>SNAMKKFSVVIAGGGSTFTPGIVLMLLANQDRFPLRSLKFYDNDGARQETIAEACKVILKEQAPEIEFSYTTDPQAAFTDVDFVMAHIRVGKYPMREQDEKIPLRHGVLGQETCGPGGIAYGMRSIGGVLELVDYMEKYSPNAWMLNYSNPAAIVAEATRRLRPNAKILNICDMPIGIEGRMAQIVGLKDRKQMRVRYYGLNHFGWWTSIEDLDGNDLMPKLREYVAKYGYVPPSNDPHTEASWNDTFAKAKDVQALDPQTMPNTYLKYYLFPDYVVAHSNPERTRANEVMDHREKNVFSACRAIIAAGKSTAGDLEIDEHASYIVDLATAIAFNTQERMLLIVPNNGAIHNFDADAMVEIPCLVGHNGPEPLTVGDIPHFQKGLMSQQVAVEKLVVDAWEQRSYHKLWQAITLSKTVPSASVAKAILDDLIAANKDYWPELH[2x]

Here, we report the deposition of 14 structures of enzymes from both the core and accessory genomes of sequence type 23 (ST23) K1 hypervirulent K. pneumoniae. Targets were selected using a shotgun approach aimed at uncharacterized metabolic proteins from ST23 K1 hypervirulent K. pneumoniae. In silico multilocus sequence typing of all K. pneumoniae isolates was completed using Kleborate. This analysis showed that 64 of the selected proteins are part of the K. pneumoniae core genome, defined as genes present in at least 95% of all strains; the other 132 proteins are part of the K. pneumoniae accessory genome and are overrepresented in the highly virulent hvKp clonal group CG23, which contains ST23 (7). Thus, the x-ray crystal structures presented here provide the basis for functional analysis of 12 uncharacterized proteins associated with high-risk K. pneumoniae infection.

Of these targets, 34 were successfully purified from large-scale preparations and entered crystallization trials. Fourteen structures were determined for 13 different targets as detailed in Fig. 1.4-[(thiophen-2-yl)methyl]benzoic acid | C12 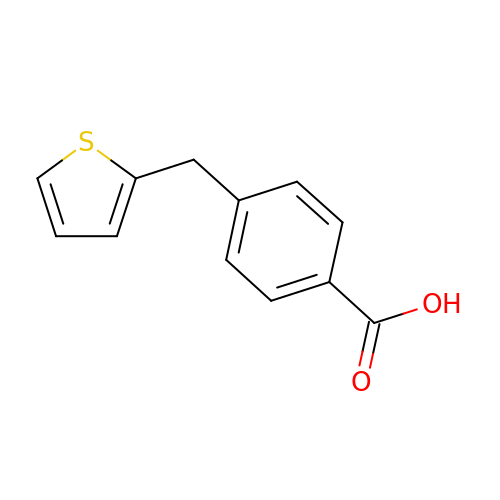H10 O2 S | OAIBKSRZDOMJKZ-UHFFFAOYSA-N>[4x]MSTSDDIHNTTATGKCPFHQGGHDQSAGAGTTTRDWWPNQLRVDLLNQHSNRSNPLGEDFDYRKEFSKLDYYGLKKDLKALLTESQPWWPADWGSYAGLFIRM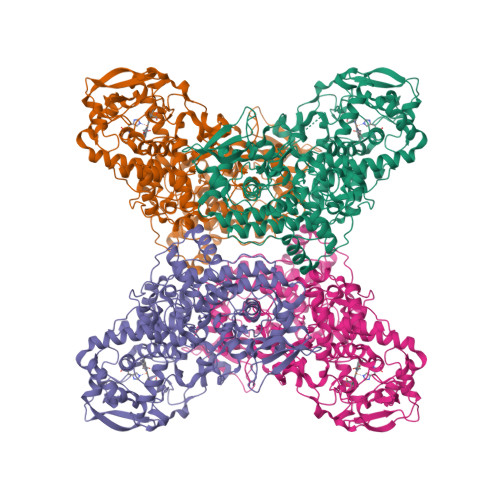AWHGAGTYRSIDGRGGAGRGQQRFAPLNSWPDNVSLDKARRLLWPIKQKYGQKISWADLFILAGNVALENSGFRTFGFGAGREDVWEPDLDVNWGDEKAWLTHRHPEALAKAPLGATEMGLIYVNPEGPDHSGEPLSAAAAIRATFGNMGMNDEETVALIAGGHTLGKTHGAGPTSNVGPDPEAAPIEEQGLGWASTYGSGVGADAITSGLEVVWTQTPTQWSNYFFENLFKYEWVQTRSPAGAIQFEAVDAPEIIPDPFDPSKKRKPTMLVTDLTLRFDPEFEKISRRFLNDPQAFNEAFARAWFKLTHRDMGPKSRYIGPEVPKEDLIWQDPLPQPIYNPTEQDIIDLKFAIADSGLSVSELVSVAWASASTFRGGDKRGGANGARLALMPQRDWDVNAAAVRALPVLEKIQKESGKASLADIIVLAGVVGVEKAASAAGLSIHVPFAPGRVDARQDQTDIEMFELLEPIADGFRNYRARLDVSTTESLLIDKAQQLTLTAPEMTALVGGMRVLGANFDGSKNGVFTDRVGVLSNDFFVNLLDMRYEWKATDESKELFEGRDRETGEVKFTASRADLVFGSNSVLRAVAEVYASSDAHEKFVKDFVAAWVKVMNLDRFDLL> GGUUGCCGAAUCCGAAAGGUACGGAGGAACCGCUUUUUGGGGUUAAUCUGCAGUGAAGCUGCAGUAGGGAUAC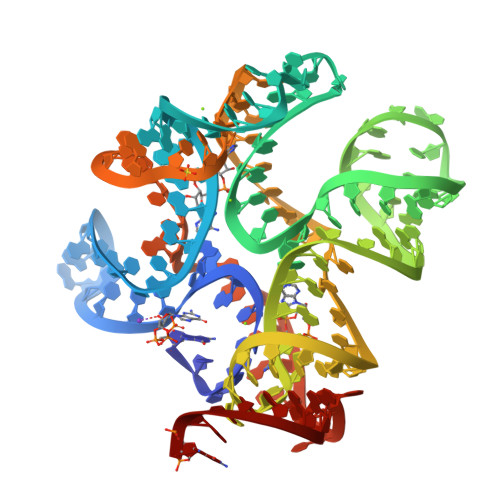CUUCUGUCCCGCACCCGACAGCUAACUCCGGAGGCAAUAAAGGAAGGAX>[4x]MDRIIQSPGKYIQGADVINRLGEYLKPLAERWLVVGDKFVLGFAQSTVEKSFKDAGLVVEIAPFGGECSQNEIDRLRGIAETAQCGAILGIGGGKTLDTAKALAHFMGVPVAIAPTIASTDAPCSALSVIYTDEGEFDRYLLLPNN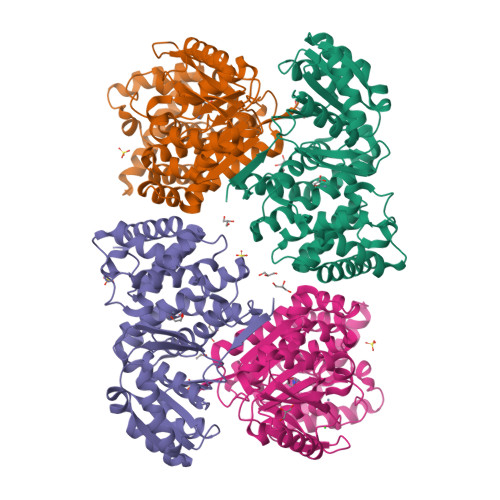PNMVIVDTKIVAGAPARLLAAGIGDALATWFEARACSRSGATTMAGGKCTQAALALAELCYNTLLEEGEKAMLAAEQHVVTPALERVIEANTYLSGVGFESGGLAAAHAVHNGLTAIPDAHHYYHGEKVAFGTLTQLVLENAPVEEIETVAALSHAVGLPITLAQLDIKEDVPAKMRIVAEAACAEGETIHNMPGGATPDQVYAALLVADQYGQRFLQEWE>MGPVWRKHYITYRINNYTPDMNREDVDYAIRKAFQVWSNVTPLK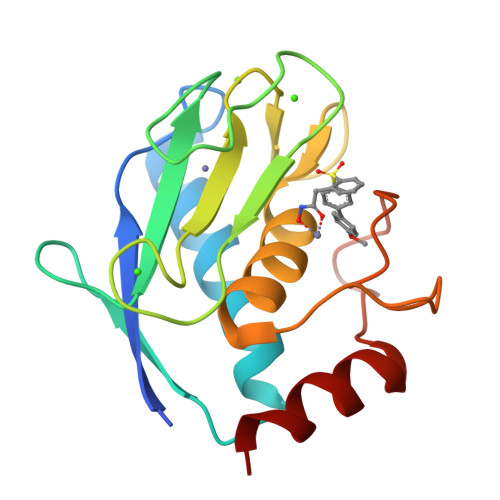FSKINTGMADILVVFARGAHGDDHAFDGKGGILAHAFGPGSGIGGDAHFDEDEFWTTHSGGTNLFLTAVHEIGHSLGLGHSSDPKAVMFPTYKYVDINTFRLSADDIRGIQSLYG[2x]> GKKSRMCGYCGAPAPYATACGLDVCVYHTHFHQHCPVIIWCGHPAGSGSCSECEPPLGKGTSPLDEVLEQVPYKPPRTVIMHVEQGLTPLDPGRYQTRRGLVSVRRGIRGNEVDLPDGDYASTALLPTCKEINMVAVASNVLRSRFIIGPPGAGKTHWLLQQVQDGDVIYTPTHQTMLDMIRALGTCRFNVPAGTTLQFPAP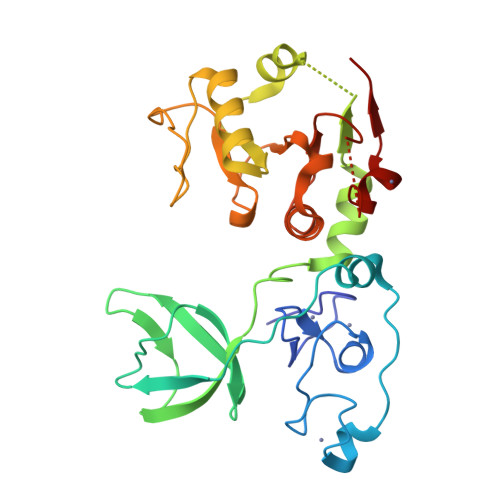SRTGPWVRILAGGWCPGKNSFLDEAAYCNHLDVLRLLSKTTLTCLGDFKQLHPVGFDSHCYVFDIMPQTQL> MNDKEKIDKFIHSNLNDDFGLSVDDLVGKVKGIGRFSAWCGNSSTKIKQVLNAVKSIGVSPALFAAYEKNEGYNGSWGWLNHTSPQGNYLTDAQFVARKLVSQSRQAGTPSWIDAGNPVDFVPASVKRKGNYDFSHNMKNGKVGRAYIPLTAAATWAAYYPEGLQASYNRVQNYGNPFLDAANTILGWGGKIDGKGGSSSGSSSSSSGTSGGLDVVARAFEEF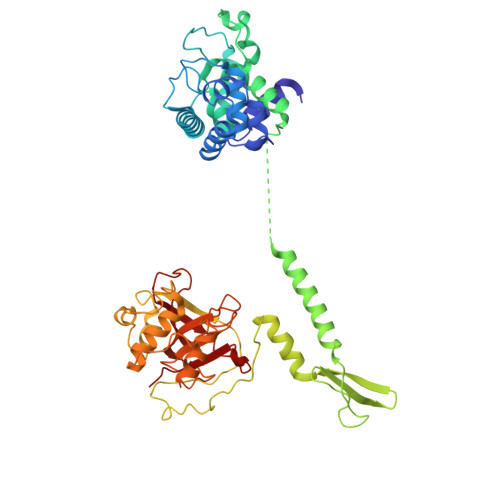LKKLQDSMQWDLHSIGTDKFFSNQMFTITKTYNNTYRLNMNQKLLDEMKDLISRIDGGSGNDTGADDSDGDHGGKAGKSVAPNGKSGRKIGGNWTYSNLPQKYKDAIEVPKFDPKYLAGSPFVNTGDTGQCTELTWAYMHQIWGKRQPAWDNQVTNGQRVWVVYRNQGARVTHRPTVGYGFSSKPNYLQAMLPGVGHTGVVVAVFKDGSFLTANYNVPPYWAPSRVVEYALIDGVPENAGDNIMFFSGIK>[4x]SLVQLWKMIFQETGKEAAKNYGLYGCNCGVGRRGKPKDATDSCCYVHKCCYKKVTGCNPKMDSYSYSWKNKAIVCGEKNPPCLKQVCECDKAVAICLRENLGTYNKKYTIYPKPFCKKADTC

Phospholipase A2 (PLA2, EC 3.1.1.4) is one of the representative toxic components of snake venom. Group II PLA2s are further categorized into several subgroups based on the amino acid at position 49. In contrast, Lys49-PLA2 lacks phospholipase activity, or exhibits minimal phospholipase activity because the catalytic Asp49 is substituted for Lys4–6. In this study, we comprehensively analyzed basic protein II (BPII), which is one of the Lys49-PLA2 homologues isolated from the venom of Protobothrops flavoviridis (PflLys49-PLA2 BPII).

The crystal structure of PflLys49-PLA2 BPII was determined at a resolution of 2.57 Å. The asymmetric unit contained four molecules of PflLys49-PLA2 BPII. These four molecules were superimposed well relative to each other with root-mean-square-deviation (r.m.s.d.) values less than 0.5 Å for the Cα-atoms. The relative orientation between molecules A and B was similar to that between molecules C and D. However, this dimer was superimposed neither on the conventional dimer nor the alternative dimer previously reported. Furthermore, basic residues were located on both sides of the interface, and the surface charges of both interfaces were positive. The area of the interface among four molecules was less than 350 Å2. Based on these observations, we concluded that the conserved relative orientation between molecules is merely preferable packing in the crystal and PflLys49-PLA2 BPII does not form any oligomers in the crystal. However, all cysteine residues formed intramolecular disulfide bonds in the crystal structure, and thus, intermolecular disulfide bond formation is highly unlikely. PflLys49-PLA2 BPII harbors seven intramolecular disulfide bonds, thus 12% of the total 122 amino acids (14 Cys residues) contributes to covalent bond formation.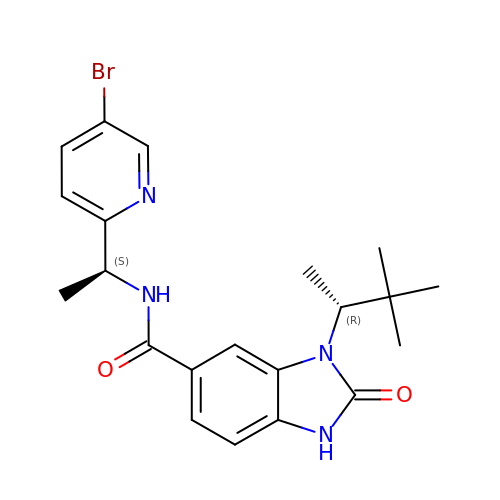N-[(1S)-1-(5-bromopyridin-2-yl)ethyl]-3-[(2R)-3,3-dimethylbutan-2-yl]-2-oxo-2,3-dihydro-1H-benzimidazole-5-carboxamide | C21 H25 Br N4 O2 | DLMZWVVEARAWSJ-QWHCGFSZSA-N FdlA from Flavobacterium sp. SA-0082 is an endo-type fucoidan-degrading enzyme that cleaves the sulfated fuco-glucuronomannan (SFGM) through a lytic mechanism. We show that the FdlA-NTD adopts a right-handed parallel β-helix fold, and possesses a substrate binding site composed of a long groove and a unique alkaline pocket. Our structural, biochemical, and enzymological analyses strongly suggest that FdlA-NTD utilizes catalytic residues different from other β-helix polysaccharide lyases, potentially representing a novel polysaccharide lyase family. Here, we report crystal structures and enzymological characterization of wild type (WT) and eight single mutants of the catalytic N-terminal domain (NTD) of FdlA, revealing its unique substrate binding pocket and identifying the key catalytic residues.

We first measured the enzymatic activity of 12 mutants and found that eight of them (D137A, K141A, H176A, F179A, E236A, R240A, Y242A, and Y242F) almost completely abolished their activities, H279A mutant retained approximately 65% of the activity compared with WT, while mutations of Asn243, Arg272, and Tyr322 to Ala only negligibly affect their activities. Brønsted base is responsible for proton extraction from C-5 atom in β-elimination reaction. Two positively charged residues Lys141 and Arg240 have their side chains pointing closely to the C-5 atom at the +1 subsite, hence are potential candidates for a catalytic base. Our structures showed that the K141A mutant possesses an active site almost identical to the WT, similar to the Y242F mutant. In contrast, Lys141 possibly functions as a catalytic base by capturing a proton from the C-5 atom at +1 subsite. Subsequently, abstraction of the proton occurs on C-5, a process that is presumably accomplished by Lys141, leading to the formation of an enolate intermediate. While it remains considerably challenging to unambiguously identify residues responsible for proton abstraction and transfer without structures of FdlA-NTD in complex with substrates or products, we were able to infer from our crystal structures and docking models that Tyr242 and Lys141 serve as the potential Brønsted acid and base, respectively. We found that the inactive FdlA-NTD mutants exhibited similar Kd values as the wild-type form. These binding assay data clearly demonstrated that while our inactive mutants lost their catalytic activity, they maintained their substrate binding ability.

> HHHHHHSSGLVPRGSHMQTTTVYSLEDLLPYLKQDNVDVKLAPGTYNVNGFDVGEDRLFSTTPLFLFEGSNSTYDFTDVKLNINTVVLTKFGNNEVNEIQILGNNNVLKNLKLEDIGTTAPSNRAQSIVIDGRDNRIEGFHLTIRGSYPYGYGDAFGAGGGSVINHRKHSGVLIRGLRNHLKDCTIISRSYGHIVFMQAASYPTVEGCYIEGEMRSTDDMLAEEGTGSPADKVDFMTVWGYKLPAGYMMSLQEGGIRAYNAGTTYIDGVEIQRATDNPTVLNCTIKNARTGVTLAHANGTKYVEGCTVLGCENGYSIGSGTVVNCGADAIYGPVFKNTYGSDKGYNADITILPPSDAYYNGHDAVAYIGGSNHNLTFRSEITEIPSNLKIMVSGDLQGLRVLHGSNPSQNNFAGTNIVLRNLTNFPVDLHSDSSNITVTSCDTDNITDNGTNNSIEAIDCDSD> PGDGDWAAAYKKATAALAKLSNTDKASIVTGVGWEKGPCVGNTAAVASIGLPELCYQDGPLGIRFVQNVTAFPTGIQTASTWDISLIYSRGLALGQEAKALGINVQLGPVAGPIGKIPEAGRNWEGFSPDPYLNGLAMSNTITGMQDAGVQACAKHFIGNEQETNRDTMSSNIDDRTFHELYLWPFADAIKANVASIMCSYNKFNETYACENNFLTTILKGELDFQGFVVSDWAAQHTTIGSANAGLDVAMPGDNFGDNYYLWGSNLLAAISNGTVAQSRLDDMVTRILASWYFVGQDQGYPAVTWSSWNGGLGGPNVQADHKQVARAIARDGIVLLTNKNKALPLKKPASLAIIGQDAIDNPAGINSCSDRGCDTGHLAMGWGSGTADFPYLVAPLDAITPLAQAQGTKLVLSTTDSTSAAASAAAAAETAIVFITADSGEGYITVDGQLGDRNSLAPWNNGTALVQAVASASKNVIVVINSVGPLILEDILALSSVKAIVWAGVSGQESGNGLADILYGSVSPSGKLPYTIAKQASDYGT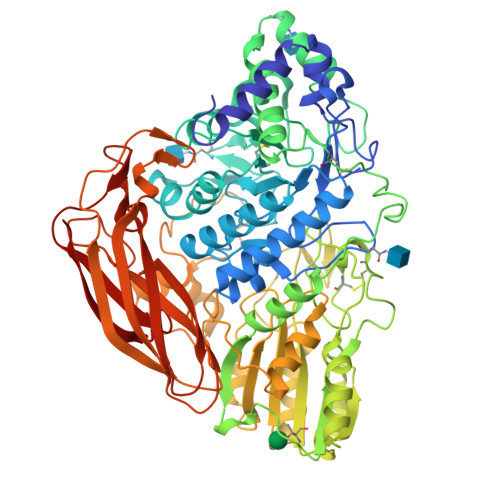AIVPGDDNFPEGLFVDYRHFDQANIQPRFEFGYGLSYTTFQYSQLTAKYSDTSAGSSTLAPGGPKGLYDIVATVTAKVTNSGTVSGAEVAQLYIGLPGSAPASPPKQLRGFDKISLKPGKSGTVTFNLRRKDLSYWDTASAQWVTPTSGEFSLYVGASSRDIRLQGSLKCSGQGIRKGGH>MRGSHHHHHHGSMNPAAEAEFNILLATDSYKVTHYKQYPPNTSKVYSYFECREKKTENSKLRKVKYEETVFYGLQYILNKYLKGKVVTKEKIQEAKDVYKEHFQDDVFNEKGWNYILEKYDGHLPIEIKAVPEGFVIPRGNVLFTVENTDPECYWLTNWIETILVQSWYPITVATNSREQKKILAKYLLETSGNLDGLEYKLHDFGYRGVSSQETAGIGASAHLVNFKGTDTVAGLALIKKYYGTKDPVPGYSVPAAEHSTITAWGKDHEKDAFEHIVTQFSSVPVSVVSDSYDIYNAC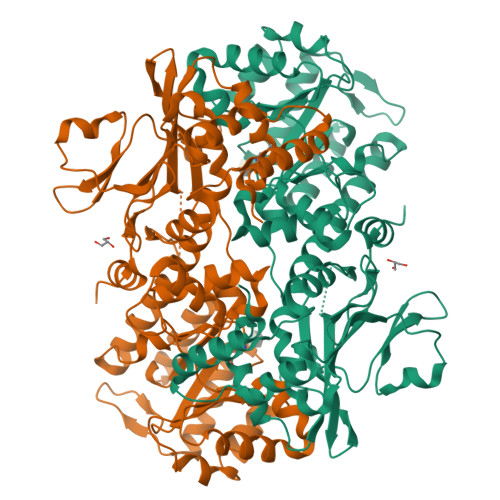EKIWGEDLRHLIVSRSTQAPLIIRPDSGNPLDTVLKVLEILGKKFPVTENSKGYKLLPPYLRVIQGDGVDINTLQEIVEGMKQKMWSIENIAFGSGGGLLQKLTRDLLNCSFKCSYVVTNGLGINVFKDPVADPNKRSKKGRLSLHRTPAGNFVTLEEGKGDLEEYGQDLLHTVFKNGKVTKSYSFDEIRKNAQLNIELEAAHH[2x]> MANKESEQNGLEAISGDIEKLSSNVDLFSKAMDDKYKELTARFDGQKSDSEEIRKAAEQATKEYAELSAKHQFFTEELVAMKARLDSPIMRSQADLDDHDRKTAIQLQRNMHEFRGGDPKEFVADESNLVDLKAYRSAVRKMLKVGIESKERVISSMTDVERKAFEASTIGPAFFTPQVLALEVDCNIECASLLDLYGQIEVSRSTFTYMKIADYGQLGEYTCDAKCDAEFGEPGNIRHLEGKTYDYRGVFCFNRKNLQEANYDFLSFMIGAAQRSHRINRNRALMVGDGINEPKGWLKEDCFPTFLTLPVNTGTPENPVQTPAFLAQDWRRFVTSFPAE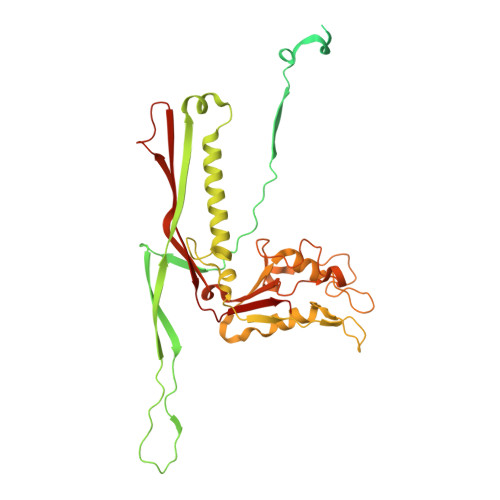YGDARSVMHQNVFGYLAAMVDANGRFLFGDGDLTFSPDLVRERIRISNCLPDPTEGNTKGGTGQDAFAAGSFIAAQAAWKTAYYAVEKRPMFFEQYEGGSSAWCVKYQFGAEDGGFVGCCEHGRVLRIG> GGSEAVSDIYKPFWEWAAKTIKERLGDDLVSYPIPDGYLRKEAMVGKGKRESLAWTQSYGYQTKKMRQIRAAHVNGGASLQVLNLVFFPHMNYDLPFLGLDLVTLPGGHLIAIDMQPLFQTEEYKKKYAEPCMDMYQKHVKNLPWGGDFPEEAKQYFSPVFLWTRPQEDKQVETYVFEAFKDYINKYLDFVEAAKPVTDPDHLARIRERQLSYLQYRAEKDPARGMFTRMYGPEWTERYIHGFLFDLEEKMESGEYKTGELLPCSDPLNFQPTPL

BV IXα is then the substrate for many members of the ferredoxin-dependent bilin reductases (FDBRs) that catalyze a regio- and stereospecific reduction of the tetrapyrrole pigment. However, during the reaction, a second aspartate residue gets involved and likely serves as a proton donor for the proton coupled electron transfer to the A-ring of the tetrapyrrole molecule. This reaction catalyzed by PebB is a formal reduction of the 2,3,31,32-dien system of the A-ring of 15,16-DHBV. Here we solved the crystal structure of the PebB homolog PEBB (nuclear encoded proteins in eukaryotes are denoted with capital letters by convention) from the eukaryotic cryptophyte alga Guillardia theta. The eukaryotic mGtPEBB is a globular single domain protein that shows the characteristic FDBR α/β/α-sandwich fold with a central antiparallel β-sheet, flanked by α-helices.

Therefore, we designed an expression construct for a truncated version of GtPEBB lacking the first 83 amino acids, which were annotated as chloroplast transit peptide by ChloroP. Incidentally, this construct contains the full FDBR domain and reflects the mature GtPEBB (mGtPEBB). Crystals of mGtPEBB diffracted slightly better, showing the same space group (P62) and almost identical unit cell parameters. The structure of mGtPEBB was refined at 1.9 Å resolution to an R factor of 21.1% and a free R factor of 23.2%. The first three residues (two residues of the linker peptide used in the expression construct, one residue of the mature protein) and residues 45–48 and 147–151 have been omitted because of missing or weak density. When comparing the substrate-free and the substrate-bound GtPEBB structures, only minor conformational changes are observed upon DHBV binding. Both models superimpose nearly perfectly, showing a root-mean-square deviation of 0.31 Å (PyMOL super, 217 Cα atoms). Substrate binding mostly leads to a stronger coordination of the mobile residues between helix H3 and β-strand S7, forming the “lid” of the active site. These residues could not be modeled reliably in the substrate-free structure but showed defined density in the substrate-bound structure. A second function is the strong coordination of the catalytically important residue Asp-219 by a salt bridge, present in both the substrate-free and DHBV-bound state.> NECISVKGRIYSILKQIGSGG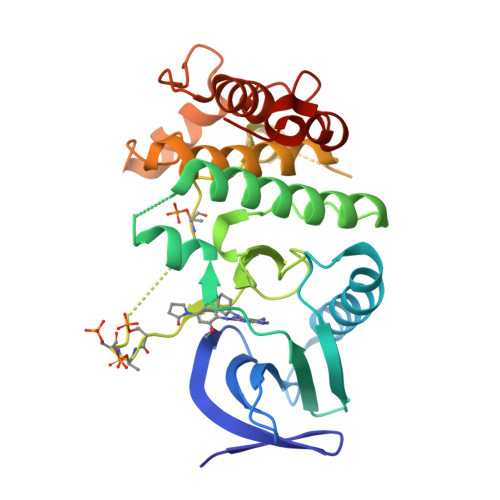SSKVFQVLNEKKQIYAIKYVNLEEADNQTLDSYRNEIAYLNKLQQHSDKIIRLYDYEITDQYIYMVMECGNIDLNSWLKKKKSIDPWERKSYWKNMLEAVHTIHQHGIVHSDLKPANFLIVDGMLKLIDFGIANQMQPDTTSVVKDSQVGTVNYMPPEAIKDMSSSRENGKSKSKISPKSDVWSLGCILYYMTYGKTPFQQIINQISKLHAIIDPNHEIEFPDIPEKDLQDVLKCCLKRDPKQRISIPELLAHPYVQIQTL>GSHMASFNRGILVAS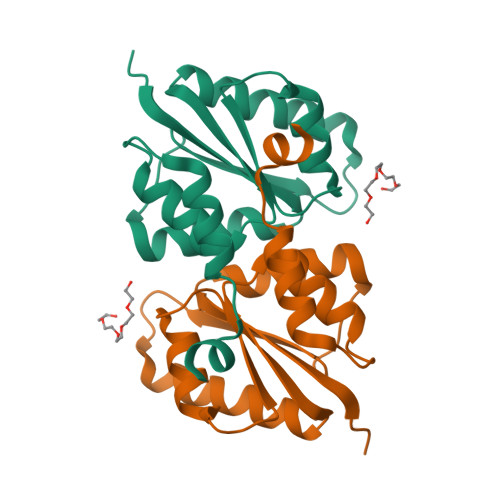HGNFASGALMTAEMFVGETTNDRVRTLGLMPGENIVEFEHYFKNQVDELLDSNQEVIVLTDLIGGSPNNVALSRFLNLDSVDIVTGFNIPLLVELISSYDSKINLEEIVHNAQNSLFNVKQQLNVEEEEDLCL[2x]4-(4-methoxyphenyl)oxane-4-carboxylic acid | C13 H16 O4 | 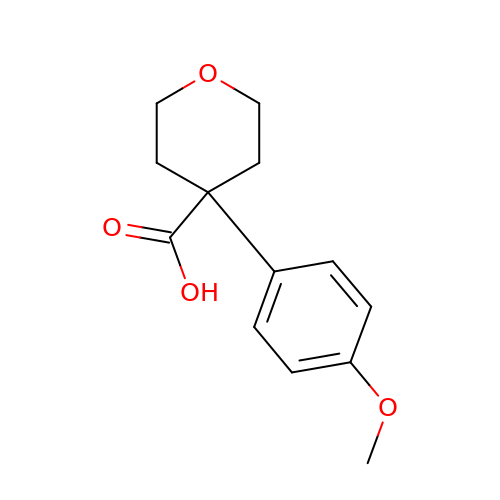HUAOQQIUUYXNFN-UHFFFAOYSA-N>FDYDGPLMKTEVPGPRSRELMKQLNIIQNAEAVHFFCNYEESRGNYLVDVDGNRMLDLYSQISSIPIGYSHPALVKLVQQPQNVSTFINRPALGILPPENFVEKLRESLLSVAPKGMSQLITMACGSCSNENAFKTIFMWYRSKERGESAFSKEELETCMINQAPGCPDYSILSFMGAFHGRTMGCLATTHSKAIHKIDIPSFDWPIAPFPRLKYPLEEFVKENQQEEARCLEEVEDLIVKYRKKKKTVAGIIVEPIQSEGGDNHASDDFFRKLRDISRKHGCAFLVDEVQTGGGSTGKFWAHEHWGLDDPADVMTFSKKMMTGGFFHKEEFRPNAPYRIFNTWLGDPSKNLLLAEVINIIKREDLLSNAAHAGKVLLTGLLDLQARYPQFISRVRGRGTFCSFDTPDESIR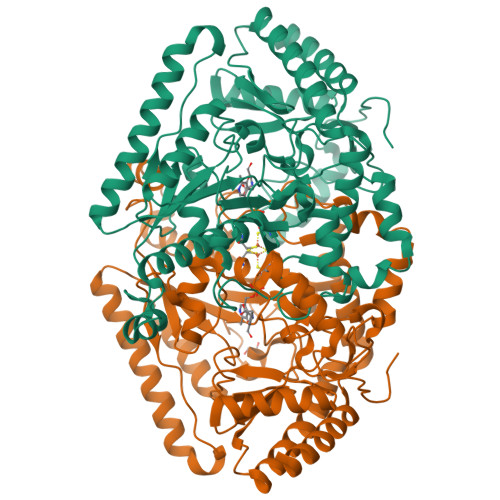NKLISIARNKGVMLGGCGDKSIRFRPTLVFRDHHAHLFLNIFSDILADF[4x]> GSMAEGSAVSDPQHAARLLRALSSFREESRFCDAHLVLDGEEIPVQKNILAAASPYIRTKLNYNPPKDDGSTYKIELEGISVMVMREILDYIFSGQIRLNEDTIQDVVQAADLLLLTDL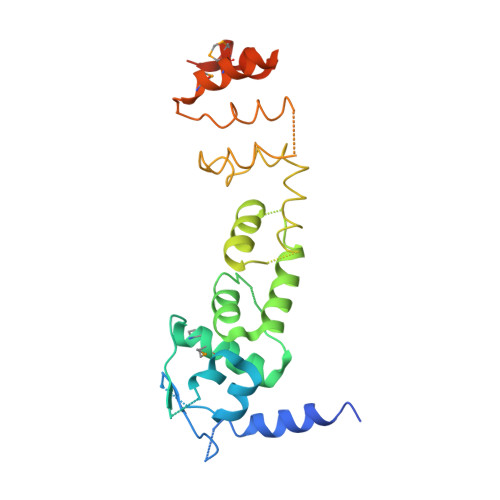KTLCCEFLEGCIAAENCIGIRDFALHYCLHHVHYLATEYLETHFRDVXXXXXXXXXXXXXXXXXXXXXXXXXXXXXXXXXXXXXXXXXXXXXXKVHMKDVMSALWVSGLDSSYLREQMLNEPLVREIVKECSNIPLS> MSRQANRGTESKKMSSELFTLTYGALVTQLC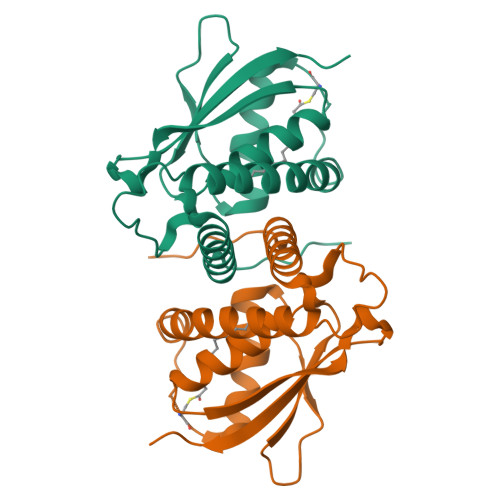KDYENDEDVNKQLDRMGYNIGVRLIEDFLARSNVGRCHDFRETADVIAKVAFKMYLGITPSITNWSPAGDEFSLILENNPLVDFVELPDNHSALIYSNLLCGVLRGALEMVQMAVEAKFVQDTLKGDGVTEIRMRFIRRIEDNLPAGEE> AAQTNAPWGLARISSTSPGTSTYYYDESAGQGSCVYVIDTGIEASHPEFEGRAQMVKTYYYSSRDGNGHGTHCAGTVGSRTYGVAKKTQLFGVKVLDDNGSGQYSTIIAGMDFVASDKNNRNCPKGVVASLSLGGGYSSSVNSAAARLQSSGVMVAVAAGNNNADARNYSPASEPSVCTVGASDRYDRRSSFSNYGSVLDIFGPGTDILSTWIGGSTRSISGTSMATPHVAGLAAYLMTLGKTTAASACRYIADTANK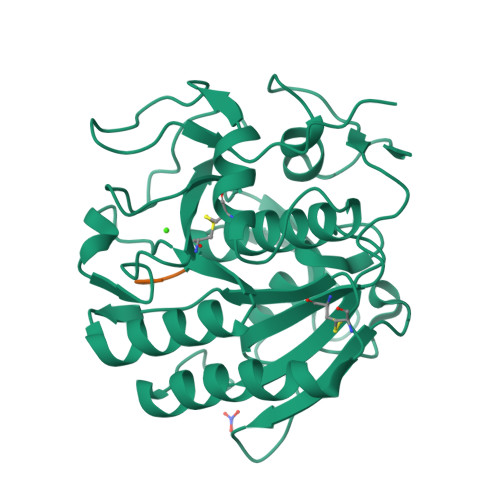GDLSNIPFGTVNLLAYNNYQA;> GALAG>[2x]GPMKTEMKDDFAKLEEQFDAKLGIFALDTGTNRTVAYRPDERFAFASTIKALTVGVLLQQKSIEDLNQRITYTRDDLVNYNPITEKHVDTGMTLKELADASLRYSDNAAQNLILKQIGGPESLKKELRKIGDEVTNPERFYPELNEVNPGETQDTSTARALVTSLRAFALEDKLPSEKRELLIDWMKRNTTGDALIRAGVPDGWEVADKTGAASYGTRNDIAIIWPPKGDPVVLAVLSSRDKKDAKYDDKLIAEATKVVMKALNMNGK

β-lactamases inactivate β-lactam antibiotics by hydrolyzing and “opening” their signature β-lactam ring. In serine-based β-lactamases of Class A, C and D, this hydrolytic process is executed in the deacylation step involving an activated water molecule carrying out nucleophilic attack on the enzyme-substrate acyl adduct ES*. Here we report structural and computational studies of Class A β-lactamase PenP with Glu166Tyr mutation that analyze the interactions between this critical water molecule, termed WAT_Nu, and other components of the active site during a full cycle of hydrolysis. In summary, by analyzing the reaction intermediates observed in the active site of a Class A β-lactamase hydrolyzing a β-lactam substrate, our study has uncovered critical features within the active site that coordinate and activate the water molecule for hydrolysis.

We set out to capture structures for in crystallo deacylation reaction intermediate by transferring cephaloridine-soaked Glu166Tyr crystals into cephaloridine-free buffer for 1, 3 or 6 seconds and then flash-freezing for x-ray data collection. Notably, the deacylation_3s structure reveals two distinct conformations in the active site. In one of the two Glu166Tyr molecules in the asymmetric unit, both WAT_Nu and Glu166Tyr are shifted back toward ES*, occupying positions similar to those observed in the apo structure. Under this new conformation, WAT_Nu re-establishes hydrogen bond with Ser70 and is positioned within ~2.3 Å away from the carbonyl carbon of ES*on the right trajectory for nucleophilic attack. In this “attack” conformation, the Bürgi–Dunitz (BD) angle of the approaching trajectory, i.e. defined as the WAT_Nu-C-O angle, is ~100°. Unexpectedly, for the other Glu166Tyr molecule in the asymmetric unit, an alternative conformation with the carbonyl of ES* tilted almost 90° upward and away from the amide group of Ala237 of the oxyanion hole. In this “tilted” conformation, WAT_Nu forms a strong hydrogen bond directly with the carbonyl oxygen of ES* across a short distance of only ~2.3 Å, locking itself into a conformation not suitable for nucleophilic attack. In summary, our QM/MM results suggest that the “attack” conformation is catalytically competent with favorable potential energy profile that matches experimental data. In contrast, the “tilted” conformation with strong hydrogen bond between WAT_Nu and the tilted carbonyl oxygen is not catalytically competent.> AEETSFVFSKFKPLEPNLILQGDALVTVAGVLQLTNVDSNGVPEPSSLGRATYSAPINIWDSATGLVASFATSFRFTIYAPNIATIADGLAFFLAPVASAPDSGGGFLGLFDSAVGDTTYQTVAVEFDTYENTVFTDPPY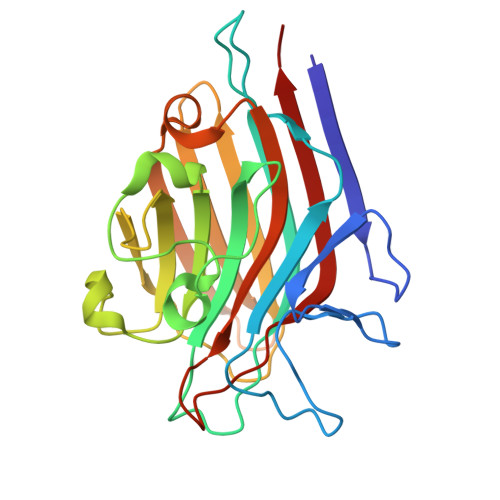THIGFDVNSISSIKTVKWSLANGEAAKVLITYNSAVKLLVASLVYPSSKTSFILADIVDLSSVLPEWVRVGFSAATGASKGYIETHDVFSWSFASKLAG Here, we explain the mechanism by which the phage AR9 non-virion RNAP (nvRNAP), a bacterial RNAP homolog, recognizes the −10 element of its deoxyuridine-containing promoter in the template strand. The AR9 sigma-like subunit, the nvRNAP enzyme core, and the template strand together form two nucleotide base-accepting pockets whose shapes dictate the requirement for the conserved deoxyuridines. The catalytically active AR9 nvRNAP core enzyme consists of four proteins that, when pairwise concatenated, show about 20% sequence identity and cover the entire lengths of the universally conserved β and β′ subunits of bacterial RNAPs. Promoter-specific transcription is performed by a five-subunit holoenzyme that, in addition to the nvRNAP core, contains the product of AR9 gene 226 (gp226).

The structure of the promoter complex has been determined by both X-ray crystallography and cryo-EM to resolutions of 3.38 and 3.80 Å, respectively. In the most populous class of the cryo-EM reconstruction and in both available crystal forms of the AR9 nvRNAP promoter complex (i.e., AR9 nvRNAP-Pro-cryoEM and AR9 nvRNAP-Pro-Xray), the enzyme bound not one but two copies of the P077 promoter-containing forked oligonucleotide—the downstream copy (as designed) and (fortuitously) the upstream one—resulting in a superstructure that resembles the complete transcription bubble found in open complexes formed by other RNAPs. Moreover, in crystallo the nvRNAP molecules and the oligonucleotides formed a train in which the upstream and downstream oligonucleotides belonging to two neighboring unit cells pi-stacked and formed a continuous double helix. Considering that the X-ray structure of the AR9 nvRNAP promoter complex is more complete, has higher resolution, and is very similar overall to the cryo-EM-derived promoter complex structure, the former is used below for the description of various structural features of the enzyme such as the conformation of the active site and the folds of various domains. The structure of the −10-like 3′-−11UUGU−8-5′ template strand promoter motif is fully resolved in the electron density map of the AR9 nvRNAP-Pro-Xray dataset. In this pocket, the −10U base is wedged between the side chains of gp226 I207 and βN gp105 R363, forming a stacking interaction with the latter. Its Watson-Crick interface forms hydrogen bonds with the side chain of βN gp105 K375 and with the main chain N of gp226 V206 and I207. Most importantly, the C5 atom of the −10U pyrimidine ring is only 3.9 Å away from the Cβ of V206, suggesting that a C5 position methyl group would clash with the V206 side chain. In the promoter complex, the bases of −11U and −9G form a stacking interaction such that the C5 and C6 atoms of −11U butt against the sugar-phosphate backbone of the −11UUG−9 segment, leaving no space for a C5 position methyl group.

> MDILENYVSFDEQARDINIAFDKLFGRDDISHMNNFSINKRSYYNCLDQISDDLNLVLNKYNDLAYSLLEIRYNMATKENYTHMEFYSDIERLFIKNEKLLNVISDIVEEEYDLDLNQASKGKKINIELQVTDNLNKIYLKSSVLMRILIPILCDFNCDDDINEVLVYDIFKEVIKSFDDGKKNALNKLYKIIYSRVFETKYSDVVIWTYLKNMSTDLMIIVKDYFKVIIKKIFPKLKHNSSVISYLDVVIKQKLKYLFTFKYPISYKPLKAETTDDEELSEQERMEINLLRNDQGNSIINECSIKQEIAKIKKKYNVTDEVMKEFINGRELNSIQIYLVKIYYSNKFKVNSNKNDIFYLLYGMTRELGEMNFSIIPEILSCAIAPNVRKMNNRKKLVDKIIHSDKYSYLLKSYLPIKNILDKNNVILQLMTIKNAKFMNKENKEVDFSTDHLAEEVLDMLLCI;> MDDISVIKNEDYEGSHRFLAEELLMPNANKTDGNRSTMFCSHLAQAVTLQKAEPPLVYTNFENQVGKYSTAGYRKANSNYKVIEKIYKNDYNYVLIVQDQETGEYTLFERAECEFLTEHYGFQWDNDKIDSLKKDDTIEKDTVLYKNTCYDENMNFGYGVNLNAAYFSYKNETLEDAIVISESAAKKLGTFSVNKVKVSVNTNDILLNLYGDNENYKGFPDIGEHIKNQIIASRRRFDYNTALYELKNLNEMRDSDTPFFADGKIVDIEIFSNVPEEELKVQKYNEQVLYYINKQKEFSNNVYQKLKKIVEGKDNNVSDKLLHFYNNCKMRIDENISYTYQNSKFSGFIMEFTILEEEPLNKGSKITGRYGNKGVISKILPDDQMPTVAEGRFKGLKADICLNPLGVFNRLNPSQLIEQELNWIAKFIRKDMEEAGSNEEKVSILLDFLNRVNKEETELMEEFINSLNKTELEEFLNDIIENGIPICQKPFFGNIGLDELWELYNHYDHIDYFKCEGISTPLIIGEIYMVRLKHEPHSKFSARSTSFMNLRGLPAKSKNFKEHKDLYSKTPVRIGNMEISNLSLTNEMGSIMDMLNSYSNNETNRRELIMQLLTGNPFDTNIDLSDVESGTSKILKSLFTCLGLSIDDVEEEWENKLNGKVEDEK;> MEKTYNLNDILLSNEYEKIKEDIKEEIINDMASKKVKYSNTSEFAKNDFLKDEFIDLVVDGETYEITYGNLITLLIVARPFNHFKVPMTEDLLFDLSDLKEYQNYYTTLLEHFGYSNEIKSIIKDVISELAIFSGDINVTFGNTVSIKSLIDLGNKVKRFRELLHYRLPNDEALEFNDIEAIIKKNLDEIMKILSETDNMLRYYIDSGAGINSKQFGQVLSLVGSKPDLFGKIIPYPINTSFLRGLDVRSFYINALGARKALITNYQQVRNSGYLTRKISMLLMDTKLIDLDDCGSHENNYLSINVENKDVLKRFSKRSYLNNNGELVEIDINDESLIGQVIKIPSPTTCASNEGVCRKCYGKLFDINKDLNIGMIAVLLLTDPLTQRLLSAKHLLETRSSKIDWGTNFEENFIVNRNLIYPKVYNGTVIIKEDDFKEDEETEEQVFDTFTLKSGNRFISISSPMRLFLNKDLKKQLDESFYNIEEMQFEIPLNKLDEGDSFATFIMDNNELSKPLREIKDLIETNKYIKDHNVNEVVNYFIYLLNESGINIQSVHSELIIREMMKLDDSDRTQFKNDKMPDYEIFRITDANLKGDSLSRSLLFEQVKKQLTTLDYDTFNKTKSSILDKLL;> MISNFRKFHGNKNQEKFNENLILNKENESILNYLDPICKTLEIIPEITYLGSSVEPINKVYKFNKEEKTSDIERSELQLIKMSFLIEKDDKKEEINKFIYFPKLIDSQYFIINGNRYYPIYQLLDSGTYRTNKALTLKTLLMPIVLREKKETFDDINGETHTMLNVDLDLFKSKVPFLIYFFSKFGFEGTLEYFGLQDLIHVLMKEDLDQLDEDEINDNVIFMITKNISLVVDKNFFSNKNNQIIIATLLNCFNTRIKIDKIYEKDYWVKKLGGYFTTNNSNKQEKGEGIILSFERILDEWTKKILRTEEKNKEDIYSVVRWMINNYLALVKQDNMNLANKRIRLYEYLLHPLLIKFSKGTYRVLNNRNSNKFEKIKTIFSNIQEGFLVKKIINNELLRYDNSVNSISLFTLILRYTQSGPQSPFSSNSTNNKLRGLHPSYLGRLGLTSTSAGDPGASGSLTPFLELPENSYMHFTEEPEINLNIDDISIDEVIES;> MGKKLSLIDFNEIYNEENLITRANPIENHEFSDDGIYSERIFGSYNEDDDDKDIDTIGWINIEPYYIINPILFTIIKKCIPSINKIINYQQSIDQNGENIDLTEEIGEDDYIGLVKFKDNFDDLLEKYTDKKKYQKEYDFLIENHDKIFINKLPVFSHKLRPATLLTGSKGKVLAFDEINNYYNFVIEYINQINEGVVSDDSIDLLLLPLLYNMQFYANNILTRIISEYLRGKKGFLRKNIMGSRINFSARNVITPLIGHPIDEVAMPYKTFAELYKFQLINLISKVKGINYNEALKFWEKGILGFNQELYNYMEELITKTKGGCTFLLNRNPTISIGSILYLKIGLIKKDYKDLTLGISNNLLSALSGDYDGDVLNIIPVFDNKMKEHFSLLSPQNFLVDRNNGRFNGDFDLQKDQILGIFILNN>MGHHHHHHMVLMTKPGTSDFVWNGIPLSMELNLWNIKEYSGSVAMKFDGEKITFDADIQNLSPKEPERYVLGYPEFYYGYKPWENHTAEGSKLPVPVSSMKSFSVEVSFDIHHEPSLPLNFAMETWLTREKYQTEASIGDVCIMVWFYFNNLTPGGEKIEEFTIPFVLNGESVEGTWELWLAEWGWDYLAFRLKDPVKKGRVKFDVRHFLDAAGKALSSSARVKDFEDLYFTVWEIGTEFGSPETKSAQFGWKFENFSIDLEVRE[2x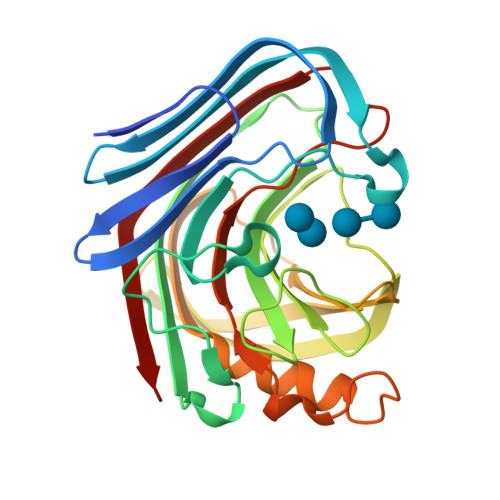]> MKFLTSN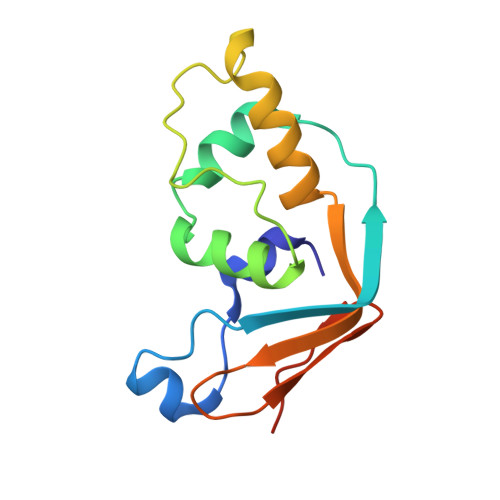FVQCASKQCVSSGNAFPLTFSALEMVQQEAEFDPEFLVSMLERIDWAALVKVANDLGNESLPDVKPEIDEPFAEGNQGLLQELHSLLIETCIVEGTMKCENCGHTYFIKNSIPNFLLPPHLAA>AGGGATCCCT[2x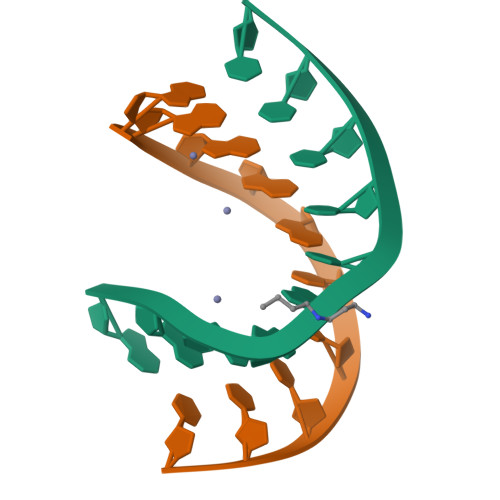]> MRRRDWCGVCLPAATLHALARRYSEYRSSYTGARSAPWAAPEAAPAYPSARSPFPLERPRFRKTHIEW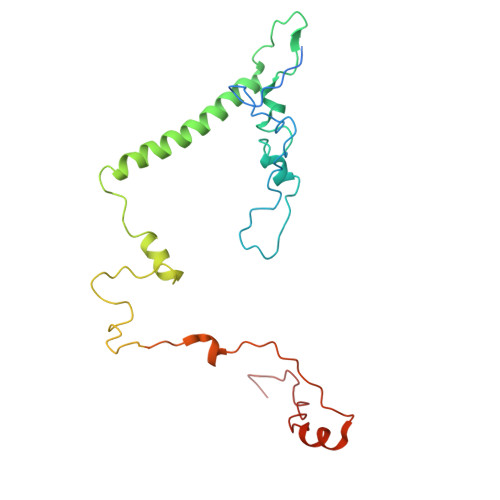MLHHGHGDRYGKYGPSREIADFEYADGTPSSISGKRFALKHHQDHLLVQLIRSAAIVERFEEEELLPRIPGTPEQRSWDPEIPLFLEDVDEFGRPPRPVAGNMVARVIEERFAQESGRTPVNLANKHAGEVLEPNTMFATYDPAAFVSDDIKKDVRRPFWSRRRWALSDNFMVPMSPKPKNTIKDE>[8x]MADALGMIEVRGFVGMVEAAD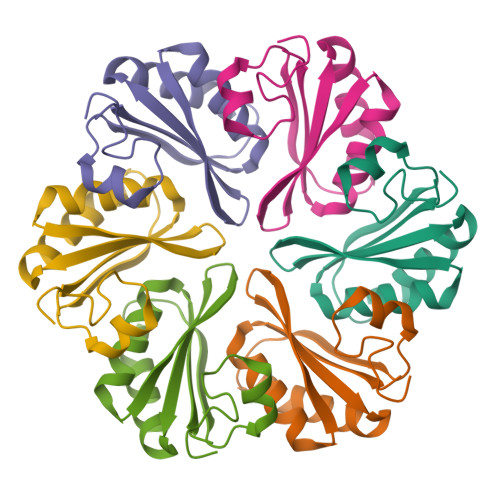AMVKAAKVELIGYEKTGGGYVTAVVRGDVAAVKAATEAGQRAAERVGEVVAVHVIPRPHVNVDAALPLGRTPGMDKSA> 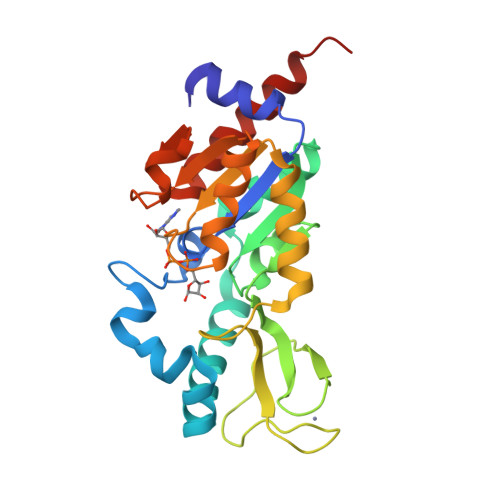MDEKLLKTIAESKYLVALTGAGVAAESGIPTFRGKDGLWNRYRPEELANPQAFAKDPEKVWKWYAWRMEKVFNAQPNKAHQAFAELERLGVLKCLITQNVDDLHERAGSRNVIHLHGSLRVVRCTSCNNSFEVESAPKIPPLPKCDKCGSLLRPGVVWFGEMLPPDVLDRAMREVERADVIIVAGTSAVVQPAASLPLIVKQRGGAIIEINPDETPLTPIADYSLRGKAGEVMDELVRHVRKALSLKLN Similar to a monorail car, they have long tunnel- or cleft-like polysaccharide-binding sites and processively hydrolyse crystalline cellulose and chitin, major types of biomass on earth, to water-soluble disaccharides. During the processive movement on crystalline chitin surface, chitinase keeps binding with single chitin chain in the catalytic cleft and repeats chemical and mechanical steps. In the chemical step, the catalytic amino acid residue and chitin N-acetyl group first cleave the glycosidic bond without attacking water, a mechanism called as substrate-assisted catalysis. From the results of this study, we conclude that SmChiA operates as a Brownian ratchet that compensates chitobiose unit interaction from the crystal surface to its binding site.

To investigate the mode of substrate binding and chain sliding, we generated an inactive mutant of SmChiA (D313A, K369M, F396A, W539A, and E540M). In this mutant, the amino acid residues constructing subsite +2 to −2 and stabilising the Michaelis complex were mutated. This mutant was designed to observe less stable substrate–enzyme complexes than the Michaelis complex. We solved four different crystal structures of the mutant bound with various lengths of oligosaccharides. These crystal structures showed that the mutant can bind to the substrate at various positions. The mutated amino acid residues were not involved in the interactions between the substrate and the enzyme in the observed intermediate complexes. We found that Glu315 showed double conformers in the crystal structure of the Sliding-intermediate (occupancy ratios of conformer A and B were 70% and 30%, respectively). The conformer A was major and interacted with the reducing end of chitohexaose via a water molecule, but the protonation state was not clear. The Trp275 should be important to relieve steric hindrance at the product-binding site during sliding motion. Next, using this Sliding-intermediate complex as an initial structure, spontaneous sliding of chitin chain was analysed in all-atom MD simulations of the wild-type enzyme.

> AAPGKPTIAWGNTKFAIVEVDQAATAYNNLVKVKNAADVSVSWNLWNGDTGTTAKVLLNGKEAWSGPSTGSSGTANFKVNKGGRYQMQVALCNADGCTASDATEIVVADTDGSHLAPLKEPLLEKNKPYKQNSGKVVGSYFVEWGVYGRNFTVDKIPAQNLTHLLYGFIPICGGNGINDSLKEIEGSFQALQRSCQGREDFKVSIHDPFAALQKAQKGVTAWDDPYKGNFGQLMALKQAHPDLKILPSIGGWTLSDPFFFMGDKVKRDRFVGSVKEFLQTWKFFDGVDIAWEFPGGKGANPNLGSPQDGETYVLLMKELRAMLDQLSVETGRKYELTSAISAGKDMIDKVAYNVAQNSMDHIFLMSYDFYGAADLKNLGHQTALNAPAWKPDTAYTTVNGVNALLAQGVKPGKIVVGTAMYGRGWTGVNGYQNNIPFTGTATGPVKGTWENGIVDYRQIAGQFMSGEWQYTYDATAEAPYVFKPSTGDLITFDDARSVQAKGKYVLDKQLGGLFSAMIDADNGDILNSMNASLGNSAGVQHHHHHH>[4x]SNAMWESKFVKEGLTFDDVLLVPAKSDVLPREVSVKTVLSESLQLNIPLISAGMDTVTEADMAIAMARQGGLGIIHKNMSIEQQAEQVDKVKRSESGGIKDIEKVIEFPNSAKDKQGRLLVGAAVGVTADAMTRIDALVKASVDAIVLDTAHGHSQGVIDKVKEVRAKYPSLNIIAGNVATAEATKALIEAGANVVKVGIGPGSICTTRVVAGVGVPQLTAVYDCATEA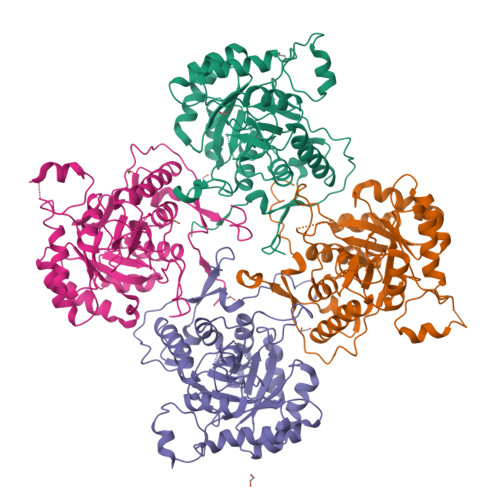RKHGIPVIADGGIKYSGDMVKALAAGAHVVMLGSMFAGVAESPGETEIYQGRQFKVYRGMGSVGAMEKGSKDRYFQEGNKKLVPEGIEGRVPYKGPLADTVHQLVGGLRAGMGYCGAQDLEFLRENAQFIRMSGAGLLESHPHHVQITKEAPNYSL5-amino-2-(6-hydroxy-3-oxo-3H-xanthen-9-yl)benzoic acid | 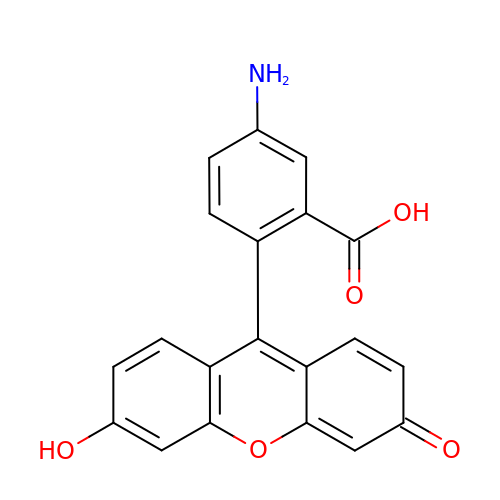C20 H13 N O5 | UTUYQGGHTUQHQQ-UHFFFAOYSA-N>[3x]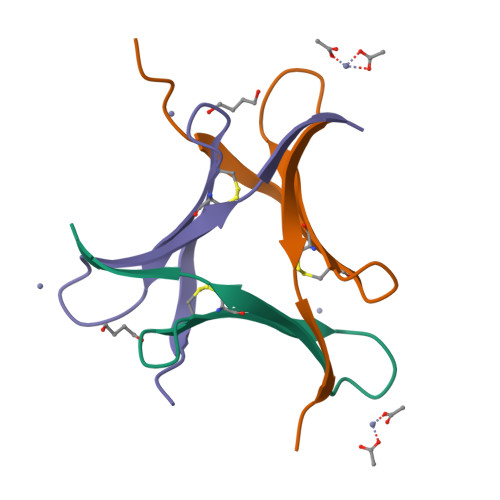GAMAPVPVTKLVCDGDTYKCTAYLDFGDGRWVAQWDTNVFHTG>[2x]MTVGNPPIHPVYAAAFAAMKERPPIHTLDLKVVRESSEARQLAANIKLPEVIEEDKVVESDGKTLKLTIVRPPGTEDQILPVLIFLHGGGFVFGSKYTHIKPVRDLTVKANVVTVFVDYSLSPEAKFPTAIEEIYAAILWVRENASSLNINAEALAVAGDSAGATLSAAVSIY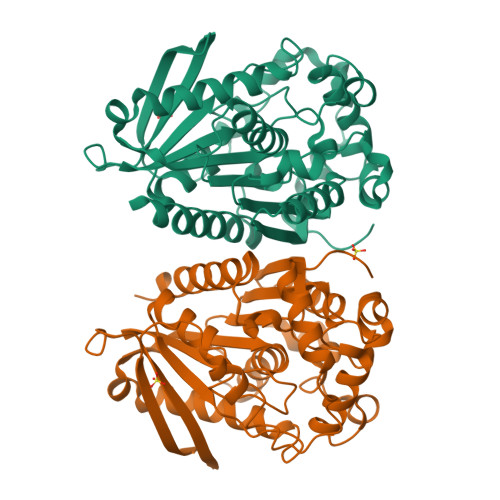AKEKGLSAAIKTQVLIYPATAVSHAKYESYKLFGNGDYILSAEDLKFFSNAYLPAPASELNDKLATLELATKADLEGLPPALLFTAESDVLRDEGEKYAQQLAEAGVDVAAVRVLGAVHGFITVPVETPQYRFTINTIVAHLRDIYAKYNALEHHHHHH> QFAKPEDAVKYRQSAITLMASHFGRMTPVVKGQAPYDAAQIKANVEVLKTLSALPWAAFGPGTEGGDARPEIWSDAASFKQKQQAFQDNIVKLSAAADAGDLDKLRAAFGDVGASCKACHDAYRK

Cytochromes c′ occur in methanotrophic, denitrifying and photosynthetic bacteria and have proposed roles in protection against nitrosative stress, NO trafficking during denitrification or pathogen defence. All cytochromes c′ have a 4 α-helix bundle structure containing a heme centre with a solvent exposed proximal His ligand and a buried hydrophobic distal pocket with a non-coordinated residue (Leu or Phe, rarely Met or Tyr) in a position to exert steric influence on the binding of diatomic gases. Unusually, cytochromes c′ are able to utilize both heme faces (distal and proximal) as a means of discriminating NO from other diatomic gases. In order to understand the factors controlling distal versus proximal NO coordination, we have examined NO binding to AXCP variants in which the occluding distal residue Leu16 is replaced with residues that are smaller (Ala, Val), of comparable size (Ile) or larger (Phe).

All of the tertiary structures are similar to wt AXCP and only salient points concerning the heme region are discussed here. Ferrous structures show the different residues at position 16 to lie over the heme in a similar manner to that of Leu16 in wt AXCP (Fig. S4†) with the exception of L16A where the side chain is essentially truncated.Three receptor types have been highlighted: VEGFR3 (also called Flt-4) regulates lymphangiogenesis, VEGFR2 (KDR/Flk-1) is the primary proangiogenic receptor, whereas VEGFR1 (Flt-1) has been proposed as a regulator of VEGFR2. In this study, we showed the presence of a metal site at the dimer interface of X-ray structures of human VEGFR1 domain 2 (hVEGFR1d2) solved in the presence of different divalent metal ions. The three structures are similar and reveal a homodimer with interlocked hydrophobic surfaces buried at the interface and a divalent cation chelated by four histidine residues (two from each monomer). Importantly, the dimer interface involves residues that lie in the core of the hVEGFR1d2 surface that interacts with VEGF-A, VEGF-B or PlGF.

The Cu2+ had a tetrahedral coordination similarly to Zn2+. Three additional Cu2+ ions were also bound to the His214 and to the N-terminal main-chain of an adjacent molecule in the crystal packing. The metal ion coordination site is octahedral for Co2+ and tetrahedral for Zn2+ and Cu2+. However, the analysis of non-redundant structures shows that the coordination of Cu2+ by three or four His residues is highly frequent and that such coordination is scarce for Co2+ and Zn2+. The mean estimation for ΔG dissociation was 12.7 kcal.mol-1, 58.1 kcal.mol-1 and 18.4 kcal.mol-1 for (hVEGFR1d2)2-Co2+, -Zn2+, and -Cu2+ respectively. Because the competition assay results indicated a higher effect of Cu2+ ions compared to Zn2+ or Co2, the Cu2+-induced dimerization of hVEGFR1d2 in solution was verified using analytical gel-filtration chromatography. In the presence of 1 mM CuSO4, two peaks were eluted corresponding respectively to the hVEGFR1d2 dimer (78% of absorption, apparent MW = 27.9 kDa) and monomer (apparent MW = 15.8 kDa). Copper (CuSO4) and palladium (Pd(OAc)2) demonstrated the lowest IC50 values (0.97 and 0.36 μM, respectively). To confirm the specific interaction of Cu2+ with hVEGFR1, the competition assay was performed in the presence of a metal chelator (EDTA, 1 eq.). Under these conditions, Cu2+ was unable to disrupt the VEGF-A/hVEGFR1-ECD interaction.

>GRPFVEMYSEIPEIIHMTEGRELVIPCRVTSPNITVTLKKFPLDTLIPDGKRIIWDSRKGFIISNATYKEIGLLTCEATVNGHLYKTNYLTHRQT[3x]> VVIANAHNEMIHDAVMDYYGKRMATCSSDKTIKIFEVEGETHKLIDTLTGHEGPVWRVDWAHPKFGTILASCSYDGKVMIWKEENGRWSQIAVHAVHSASVNSVQWAPHEYGPMLLVASSDGKVSVVEFKENGTTSPIIIDAHAIGVNSASWAPATIEEDGEHNGTKESRKFVTGGADNLVKIWKYNSDAQTYVLESTLEGHSDWVRDVAWSPTVLLRSYMASVSQDRTCIIWTQDNEQG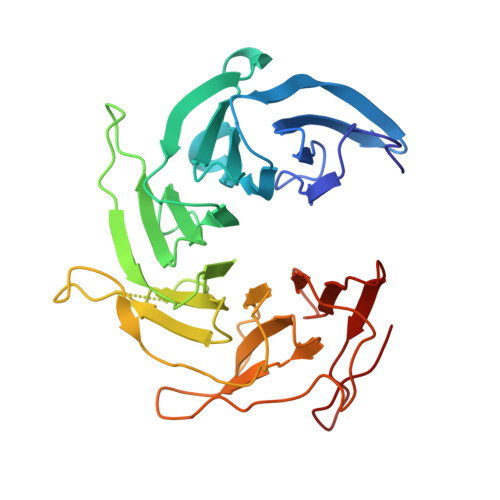PWKKTLLKEEKFPDVLWRASWSLSGNVLALSGGDNKVTLWKENLEGKWEPA>[2x]MKKFLKSTAALALGLSLTFGLFSPAQAAAPFNGTMMQYFEWYLPDDGTLWTKVANEANNLSSLGITALWLPPAYKGTSRSDVGYGVYDLYDLGEFNQKGTVRTKYGTKAQYLQAIQAAHAAGMQVYADVVFDHKGGADGTEWVDAVEVNPSDRNQEISGTYQIQAWTKF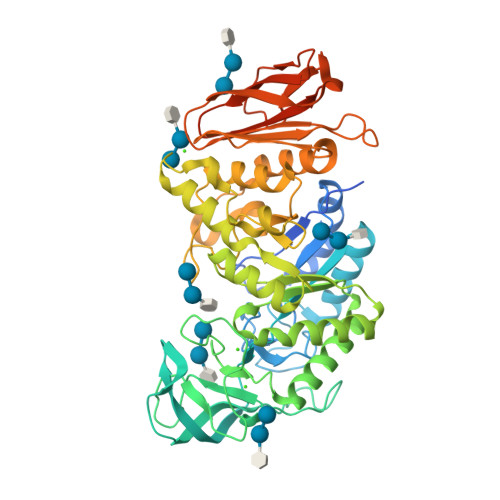DFPGRGNTYSSFKWRWYHFDGVDWDESRKLSRIYKFRGIGKAWDWEVDTENGNYDYLMYADLDMDHPEVVTELKNWGKWYVNTTNIDGFRLDAVKHIKFSFFPDWLSYVRSQTGKPLFTVGEYWSYDINKLHNYITKTNGTMSLFDAPLHNKFYTASKSGGAFDMRTLMTNTLMKDQPTLAVTFVDNHDTEPGQALQSWVDPWFKPLAYAFILTRQEGYPGVFYGDYYGIPQYNIPSLKSKIDPLLIARRDYAYGTQHDYLDHSDIIGWTREGVTEKPGSGLAALITDGPGGSKWMYVGKQHAGKVFYDLTGNRSDTVTITSDGWGEFKVNGGSVSVWVPRKTTVSTITRPITTRPWTGEFVRWTEPRLVAWP> MPLELTQSRVQKIWV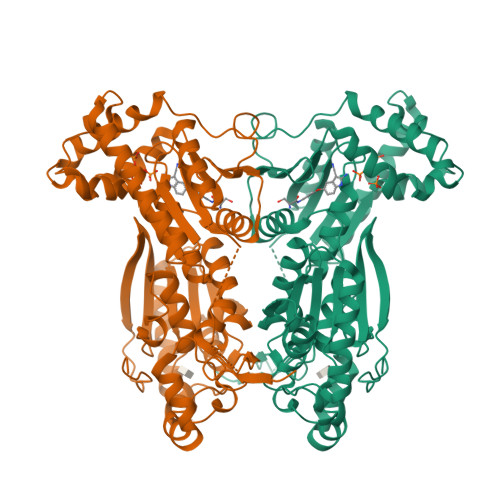PVDHRPSLPRSCGPKLTNSPTVIVMVGLPARGKTYISKKLTRYLNWIGVPTKVFNVGEYRREAVKQYSSYNFFRPDNEEAMKVRKQCALAALRDVKSYLAKEGGQIAVFDATNTTRERRHMILHFAKENDFKAFFIESVCDDPTVVASNIMEVKISSPDYKDCNSAEAMDDFMKRISCYEASYQPLDPDKCDRDLSLIKVIDVGRRFLVNRVQDHIQSRIVYYLMNIHVQPRTIYLCRHGENEHNLQGRIGGDSGLSSRGKKFASALSKFVEEQNLKDLRVWTSQLKSTIQTAEALRLPYEQWKALNEIDAGVCEELTYEEIRDTYPEEYALREQDKYYYRYPTGESYQDLVQRLEPVIMELERQENVLVICHQAVLRCLLAYFLDKSAEEMPYLKCPLHTVLKLTPVAYGCRVESIYLNVESVCTHRERSEDAKKGPNPLMRRNSVTPLASPEPTKKPRINSFEEHVASTSAALPSCLPPEVPTQLPGQNMKGSRSSADSSRKH> MTVLIIGMGNIGKKL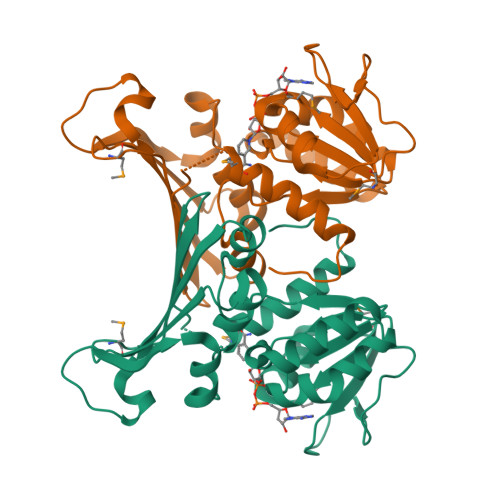VELGNFEKIYAYDRISKDIPGVVRLDEFQVPSDVSTVVECASPEAVKEYSLQILKNPVNYIIISTSAFADEVFRERFFSELKNSPARVFFPSGAIGGLDVLSSIKDFVKNVRIETIKPPKSLGLDLKGKTVVFEGSVEEASKLFPRNINVASTIGLIVGFEKVKVTIVADPAMDHNIHIVRISSAIGNYEFKIENIPSPENPKTSMLTVYSILRTLRNLESKIIFG>[2x]MGRISDKFTELKEKREKALVSYLMVGYPDYETSLKAFKEVLKNGTDILEIGFPFSDPVADGPTIQVAHEVALKNGIRFEDVLELSETLRKEFPDIPFLLMTYYNPIFRIGLEKFCRLSREKGIDGFIVPDLPPEEAEELKAVMKKYVLSFVPLGAPTSTRKRIKLICEAADEMTYFVSVTGTTGAREKLPYERIKKKVEE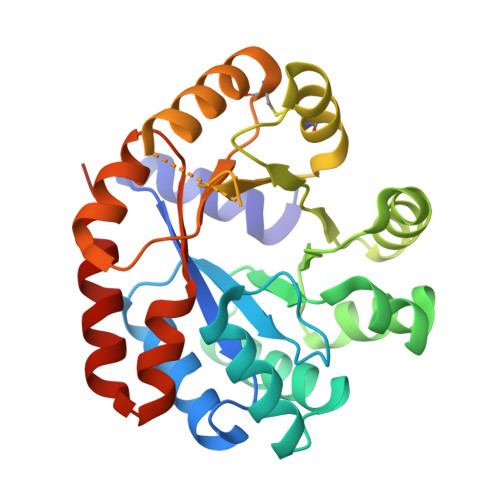YRELCDKPVVVGFGVSKKEHAREIGSFADGVVVGSALVKLAGQKKIEDLGNLVKELKEGLRE>[2x]MNVRLCYASQRNEKNEDLLQDLRDILTEARDFNDLNGICGVLYYADNAFF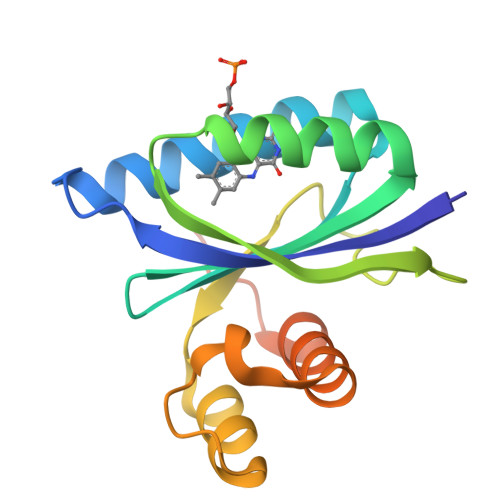QCLEGEQEVVERLFEKIQKDQRHYNIKWLCTYSIDEHSFQRWSMKYVQRNTNIETFFLNMGENTFNPLLLNQQNLKFFLNELLIAEQTKMNTVKKVGMVNRGVNPF>EERRRRAAAVIEEVEQRFSTPTALLRGIADAMVEEMERGLRADPHAPLKMLISYVDNLPTGDEHGLFYALDLGGTNFRVIRVQLGGREKRVVSQQYEEVAIPPHLMVGTSMELFDFIAAELESFVKTEGEDFHLPEGRQRELGFTFSFPVHQTSISSGTLIKWTKGFSINGTVGEDVVAELSRAMERQGLDMKVTALVNDTVGTLAGGRYVDNDVAAAVILGTGTNAAYVEHANAIPKWTGLLPRSGNMVINMEWGNFKSERLPRSDYDNALDFESLNPGEQIYEKMISGMYLGEIVRRILLKLAHDASLFGDVVPTKLEQRFILRTPDMSAMHHDTSHDLKHLGAKLKDILGVADTSLEARYITLHVCDLVAERGARLAAAGIYGILKKLGRDRVPS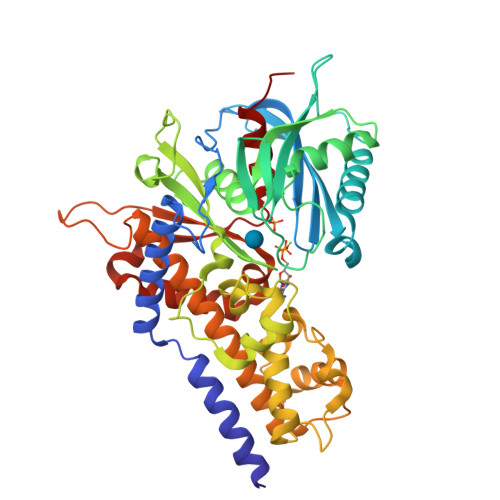DGSQKQRTVIALDGGLYEHYKKFRTCLEATLADLLGEEAASSVVVKLANDGSGIGAALLAASHSQYA[3x]>MFRKLAAECFGTFWLVFGGCGSAVLAAGFPELGIGFAGVALAFGLTVLTMAFAVGHISGGHFNPAVTIGLWAGGRFPAKEVVGYVIAQVVGGIVAAALLYLIASGKTGFDAAASGFASNGYGEHSPGGYSM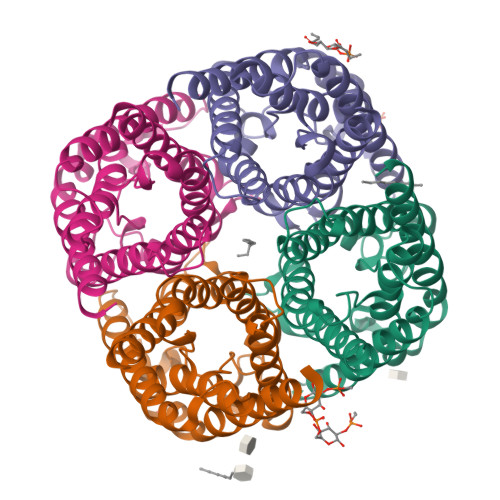LSALVVELVLSAGFLLVIHGATDKFAPAGFAPIAIGLALTLIHLISIPVTNTSVNPARSTAVAIFQGGWALEQLWFFWVVPIVGGIIGGLIYRTLLEKRD[8x]> MGELRVGLEESELWLRFKELTNEMIVTKNGRRMFPVLKVNVSGLDPNAMYSFLLDFVAADNHRWKYVNGEWVPGGKPEPQAPSCVYIHPDSPNFGAHWMKAPVSFSKVKLTNKLNGGGQIMLNSLHKYEPRIHIVRVGDPQRMITSHCFPETQFIAVTAYQNEEITALKIKYNPFAKAFLDA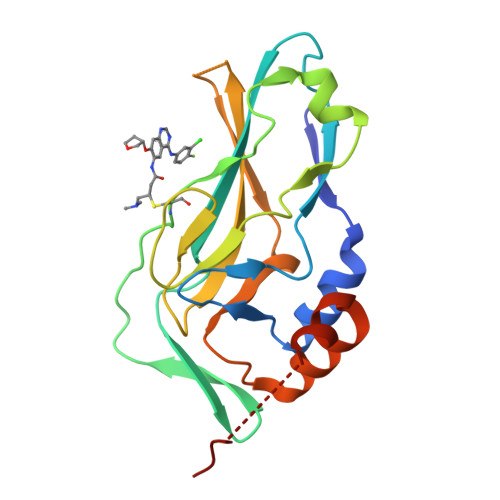KERSHHHHHH> MEDINFASLAPRHGTRPFMGTWNEIGTSQLNGGAFNWSSVWSGLKNFGSTLRTYGNKAW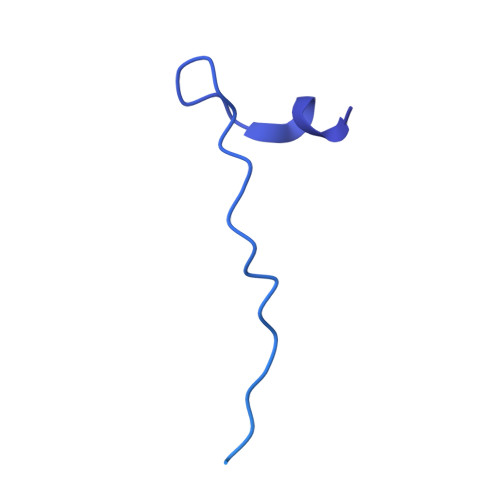NSSTGQLLREKLKDQNFQQKVVDGLASGINGVVDIANQAVQREINSRLDPRPPTVVEMEDATLPPPKGEKRPRPDAEETILQVDEPPSYEEAVKAGMPTTRIIAPLATGVMKPATLDLPPPPAPAPPKATPVVQAPPVATAVRRVPARRQAQNWQSTLHSIVGLGVKSLKRRRCY> AEEWYFGKITRRESERLLLNPENPRGTFLVRESETTKGA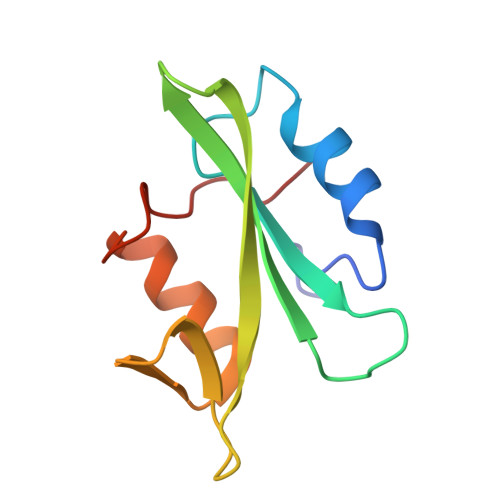YCLSVSDFDNAKGLNVKHYKIRKLDSGGFYITSRTQFSSLQQLVAYYSKHADGLCHRLTNVCP>GPMDFLRSLDWTQVIAGQYVSNPRFNISDYFEIVRQPGDGNCFYHSIAELTMPNKTDHSYHYIKRLTESAARKYYQEEPEARLVGLSLEDYLKRMLSDNEWGSTLEASMLAKEMGITIIIWTVAASDEVEAGIKFGDGDVFTAVNLLHSGQTHFDALRILPQFETDTREALSLMDRVIAVDQLTSSSSDELQDYEDLALALTSAEESNRRSSLDEVTL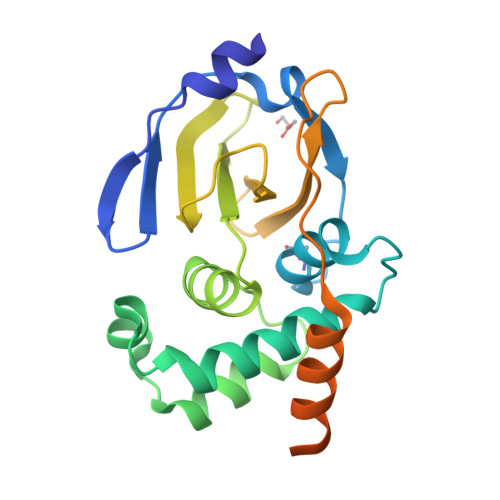S[2x]>MSYKLTYFSIRGLAEPIRLFLVDQDIKFIDDRIAKDDFSSIKSQFQFGQLPCLYDGDQQIVQSGAILRHLARKYNLNGENEMETTYIDMFCEGVRDLHVKYTRMIYMAYETEKDPYIKSILPGELAKFEKLLATRGNGRNLILGDKISYADYALFEELDVHQILDPHCLDKFPLLKVFHQRMKDRPKLKEYCEKRDAAKVPVNGNGK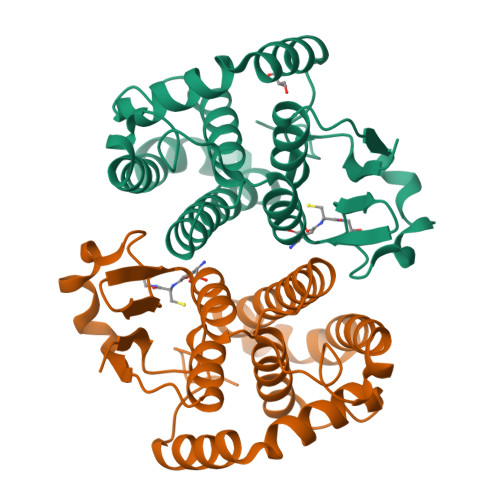Q[2x]> PHMKNKIVFAPIGQGGGNIVDTLLGICGDYNALFINTSKKDLDSLKHAKHTYHIPYAEGCGKERKKAVGYAQTYYKQIIAQIMEKFSSCDIVIFVATMAGGAGSG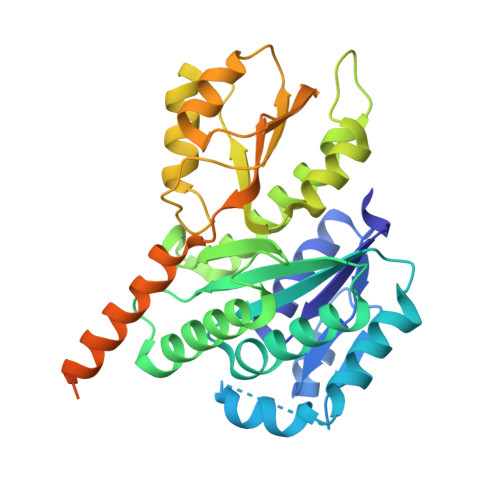ITPPILGLAKQMYPNKHFGFVGVLPKATEDIDEHMNAIACWNDIMRSTNEGKDISIYLLDNNKREKESDINKEFATLFNDFMNMSESHAEGVVDEDEISKLLTMKKSNVILEFDDKEDIQVALAKSLKESIFAEYTTNTCEFMGISTTRVVDVEAIKSIVGYPRRTFKGYNSKKNIVVATGIEPQKTTVQMMNEIIEDKMKQRREVTSKSENMIIEPIALDDEDNKSVISSNEKEISIDNVEKEIDINDFFSKYM>MGHHHHHHHHHSSGHIDDDDKHMDGLLEVVYGLLPENFPDPELAHDMVMWLAAKGYLPYDLERDDPELSVNIKGLTFHTPVGLAAGFDKNAEAPLNFCKMGFGFVEVGTITPKPQLGNPKPRIFRLAKDHAIINRCGFNSAGLDVVEPRLEKVSRDRWHDRLERHCVLGVNIGKNKDTVNAEDDIREGVKRVGRFADYLVINLSSPNTKGLRTLQQRDHLRSIITAAQSELEKLEERSRAQRERDGHSNPSEEEEAASSDSVTRKAEQFFPTQTGKRPLLFVKIAPDLTDEEKRDIADVALETGLDGLIVTNTTIQRPESLRSESKHETGGLSGRPLKAMSTKCVSDMYKMTNGQVAIIASGGIETGLDAYKRIRAGASAVEVYTSMIYRGPIVARRVKDELLNILNQAGIYNVQDAIGLDHRPPKKKRVRKPTFD[4x]

DHODH catalyzes the oxidation of dihydroorotate and the reduction of an acceptor in the fourth and rate-limiting step of de novo biosynthesis of pyrimidines, molecules that serve as building blocks for DNA and RNA and are indispensable metabolites in all living organisms. Based on localization and electron acceptor, DHODHs are classified into two families: Family 1 members are soluble proteins localized to the cytosol, while family 2 members are membrane proteins localized to the inner mitochondrial membrane. Family 2 DHODH enzymes use respiratory quinones as electron acceptors. Amongst the 6 enzymes of the de novo pathway, DHODH is the rate-limiting step and the key enzyme connecting pyrimidine biosynthesis to ETC at the level of ubiquinone.

The crystal structures of inhibitor-free EtDHODH and EtDHODH-ferulenol complex were determined at resolutions of 3.5 Å and 3.65 Å, respectively. Both crystal forms contain four EtDHODH chains per asymmetric unit. The fact that; (i) there are no significant intermolecular interactions in either crystal structure, (ii) EtDHODH migrates at similar sizes with PfDHODH and HsDHODH, i.e., around 45 kDa, in high-resolution clear native electrophoresis using dodeylmaltoside buffer (micelle size of 72 kDa) and visualized by CBB and DHODH activity staining collectively suggest that EtDHODH is functionally monomeric, consistent with other family 2 DHODHs such as those from human and P. falciparum. EtDHODH contains two domains connected by an extended loop and corresponding to a small N-terminal domain (N-terminus to Ala31) and a large C-terminal domain (Asp43 to the C-terminus). The small N-terminal domain is the enzyme’s membrane binding region, which forms two N-terminal amphiphilic helixes (αA and αB). The large domain has an α/β-barrel fold with a central barrel of eight parallel β strands (β1–β8) surrounded by eight α helices (α1–α8). The large domain of EtDHODH contains additional antiparallel β strands (βC, βD, and βE) at the top of the barrel. The long insertion region of EtDHODH (residues 218-243 in the inhibitor-free structure and residues 217-239 in the ferulenol complex structure) is missing from the final structures due to the insertion sequences’ poor electron density. In the ligand-free EtDHODH crystal structure, the electron density map of the N-terminal helix region (αA) was disordered, indicating the high flexibility of this region. The N-terminal extension found in DHODHs from other apicomplexan parasites, such as P. falciparum, T. gondii, and Neospora caninum, is not conserved in EtDHODH.>[2x]MSLIASIGELLIDLISVEEGDLKDVRLFEKHPGGAPANVAVGVSRLGVKSSLISKVGNDPFGEYLIEELSKENVDTRGIVKDEKKHTGIVFVQLKGASPSFLLYDDVAYFNM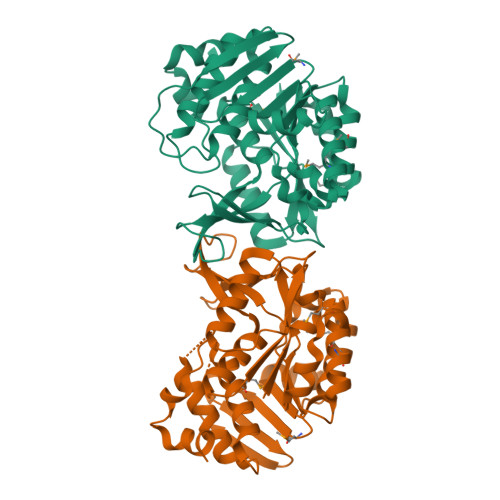TLNDINWDIVEEAKIVNFGSVILARNPSRETVMKVIKKIKGSSLIAFDVNLRLDLWRGQEEEMIKVLEESIKLADIVKASEEEVLYLENQGVEVKGSMLTAITLGPKGCRLIKNETVVDVPSYNVNPLDTTGAGDAFMAALLVGILKLKGLDLLKLGKFANLVAALSTQKRGAWSTPRKDELLKYKEAREVLAEGHHHHHH>MTGGTGADAASAGASSTRPELRGERCLPPAGPVKVTPDDPRYLNLKLRGANSRFNGEPDYIHLVGSTQQVADAVEETVRTGKRVAVRSGGHCFEDFVDNPDVKVIIDMSLLTEIAYDPSMNAFLIEPGNTLSEVYEKLYLGWNVTIPGGV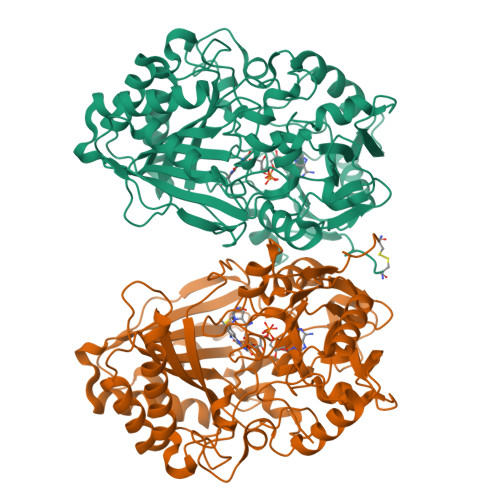CGGVGVGGHICGGGYGPLSRQFGSVVDYLYAVEVVVVNKQGKARVIVATRERDDPHHDLWWAHTGGGGGNFGVVTKYWMRVPEDVGRNPERLLPKPPATLLTSTVTFDWAGMTEAAFSRLLRNHGEWYERNSGPDSPYTGLWSQLMIGNEVPGMGESGFMMPIQVDATRPDARRLLDAHIEAVIDGVPPAEVPEPIEQRWLASTPGRGGRGPASKTKAGYLRKRLTDRQIQAVYENMTHMDGIDYGAVWLIGYGGKVNTVDPAATALPQRDAILKVNYITGWANPGNEAKHLTWVRKLYADVYAETGGVPVPNDVSDGAYINYPDSDLADPGLNTSGVPWHDLYYKGNHPRLRKVKAAYDPRNHFHHALSIRP[2x]> MAAAVAMETDDAGNRLRFQLELEFVQCLANPNYLNFLAQRGYFKDKAFVNYLKYLLYWKDPEYAKYLKYPQCLHMLELLQYEHFRKELVNAQCAKFIDEQQILHWQHYSRKRMRLQQALAEQQQQN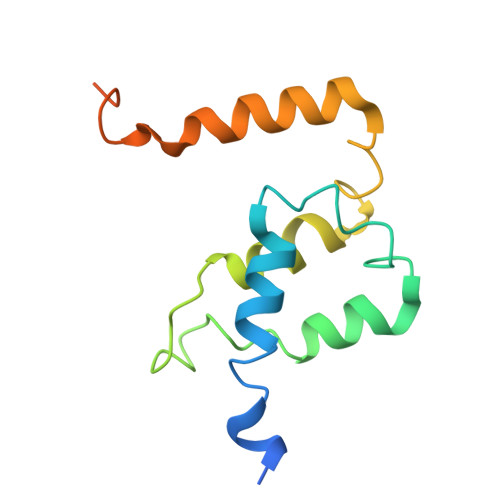NTSGK> MEDENILRNAVNLQVLKFHYPEIESIIDIASHVAVYQFDVGSQKWLKTSIEGTFFLVKDQRARVG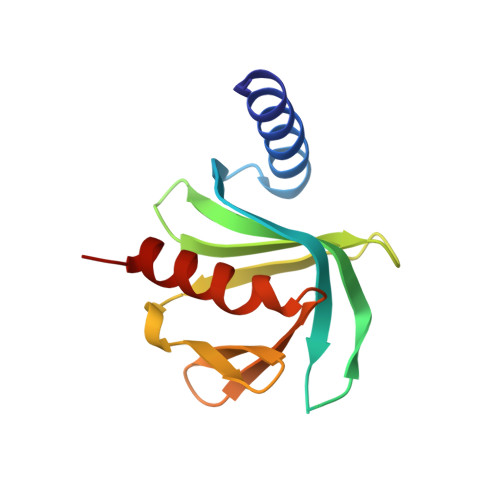YVILNRNSPENLYLFINHPSNVHLVDRYLIHRTENQHVVGLWMFDPNDMSRIFNIVKESLLR>[3x]MANAPHGGVLKDLLARDAPRQAELAAEAESLPAVTLTERQLCDLELIMNGGFSPLEGFMNQADYDRVCEDNRLADGNVFSMPITLDASQEVIDEKKLQAGSRITLRDFRDDRNLAILTIDDIYRPDKTKEAKLVFGGDPEHPAIVYLNNTVKEFYIGGKIEAVNKLNHYDYVALRYTPAELRVHFDKLGWSRVVAFQTRNPMHRAHRELTVRAARSRQANVLIHPVVGLTKPGDIDHFTRVRAYQALLPRYPNGMAVLGLLGLAMRMGGPREAIWHAIIRKNHGATHFIVGRDHAGPGSNSKGEDFYGPYDAQHAVEKYKDELGIEVVEFQMVTYLPDTDEYRPVDQVPAGVKTLNISGTELRRRLRSGAHIPEWFSYPEVVKILRESNPPRATQGFTIFLTGYMNSGKD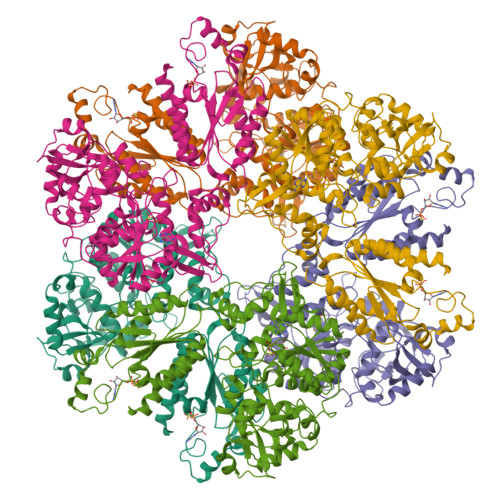AIARALQVTLNQQGGRSVSLLLGDTVRHELSSELGFTREDRHTNIQRIAFVATELTRAGAAVIAAPIAPYEESRKFARDAVSQAGSFFLVHVATPLEHCEQSDKRGIYAAARRGEIKGFTGVDDPYETPEKADLVVDFSKQSVRSIVHEIILVLESQGFLERQ> MEPLLLAWSYFRRRRFQLCADLCTQMLEKSPCDQAAWILKARALTEMVYVDEIDVDEEGIAEMILDENAIAQVPRPGTSLKLPGTNQTGGPSPAVRPVTQAGRPITGFLRPSTQSGRPGTIEQAIKTPRTAYTARPIASSSGRFVRLGTASMLTSPDGPFINLSRLNLAKYAQKPKLAKALFEYIFHHENDVKTALDLAALSTEHSQYKDWWWKVQIGKCYYRLGLYREAEKQFKSALKQQEMVDTFLYLAKVYISLDQPLTALNLFKQGLDKFPGEVTLLCGIARIYEEMNNISSATEYYKEVLKQDNTHVEAIACIGSNHFYTDQPEVALRFYRRLLQMGVYNCQLFNNLGLCCFYAQQYDMTLTSFERALSLAENEEEVADVWYNLGHVAVGTGDTNLAHQCFRLALVSNNQHAEAYNNLAVLEMRRGHVEQAKALLQTASSLA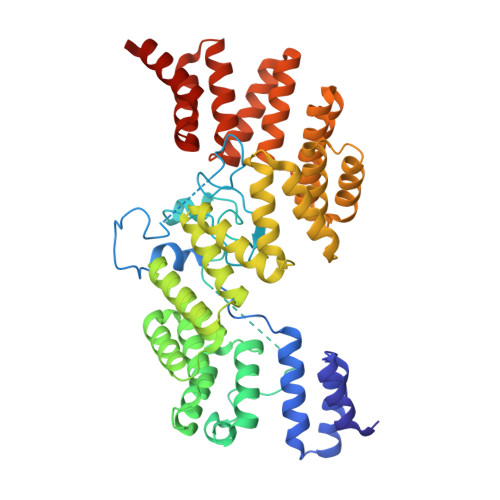PHMYEPHFNFATISDKIGDLQRSYAAAKKSEAAFPDHVDTQHLIKQLEQHFAML> MSLDWQTLLNRERLGKTLHSPEELGRSPFHKDHDRIIFSGAFRRLGRKTQVHPVSSNDHIHTRLTHSLEVSCVGRSLGMRVGETLRAALPDWCDPSDLGMVVQSACLAHDIGNPPFGHSGEDAIRNWFNQAAGRGWLDAMSETERNDFLNFEGNAQGFRVLTQLEYHQFDGGTRLTYATLGTYLKYPWTARHADSLGYKKHKFGCYQSELPILEQI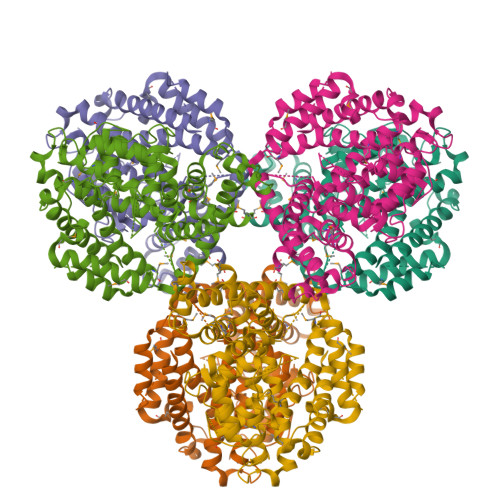AGKLGLPQLEEQRWARHPLVYLMEAADDICYALIDLEDGLEMDLLDYAEVESLLLGLVGDDLPETYRQLGPGDSRRRKLAILRGKAIEHLTNAAARAFVEQQDALLAGTLPGDLVEHMHGPAKRCVLNAKDMARKKIFQDKRKTLHEIGAYTTLEILLNAFCGAAVEQFGGRTPSFKHRRILDLLGNSAPDPKAPLHASFLRMIDFIAGMTDSYASEMAREMTGRSGEGHHHHHH>[2x]SRMQLSEEQAAVLRAVLKGQSIFFTGSAGTGKSYLLKRILGSLPPTGTVATASTGVAACHIGGTTLHAFAG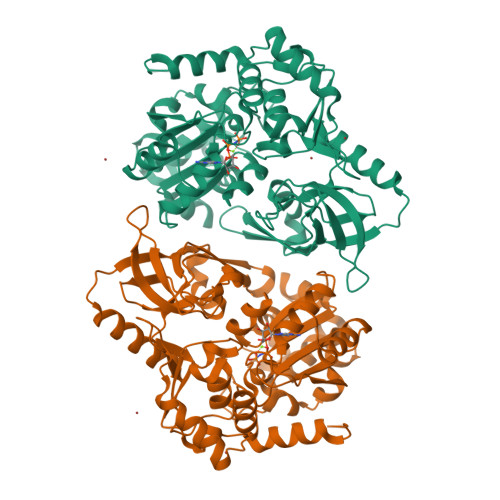IGSGQAPLAQCVALAQRPGVRQGWLNCQRLVIDEISMVEADLFDKLEAVARAVRQQNKPFGGIQLIICGDFLQLPPVTKGSQPPRFCFQSKSWKRCVPVTLELTKVWRQADQTFISLLQAVRLGRCSDEVTRQLQATASHKVGRDGIVATRLCTHQDDVALTNERRLQELPGKVHRFEAMDSNPELASTLDAQCPVSQLLQLKLGAQVMLVKNLSVSRGLVNGARGVVVGFEAEGRGLPQVRFLCGVTEVIHADRWTVQATGGQLLSRQQLPLQLAWAMSIHKSQGMTLDCVEISLGRVFASGQAYVALSRARSLQGLRVLDFDPMAVRCDPRVLHFYATLRRGRSL>GHFKDPKRLYCKNGGFFLRIHPDGRVDGVREKSDPHIKLQLQAEERGVVSIKGVSANRYLAMKEDGRLLASKSVTDECFFFERLESNNYNTYRSRKYTSWYVALKRTGQYKLGSKTGPGQKAILFLPMSAKS[2x];>[2x]TDNTKPNRMPVAPYWTSPEKMEKKLHAVPAAKTVKFKCPSSGTPQPTLRWLKNGKEFKPDHRIGGYKVRYATWSIIMDSVVPSDKGNYTCIVENEYGSINHTYQLDVVERSPHRPILQAGLPANKTV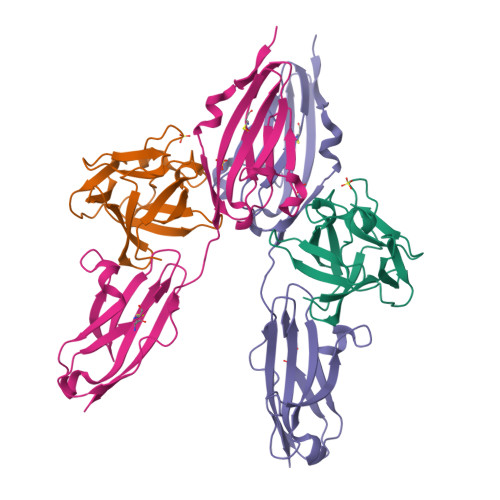ALGSNVEFMCKVYSDPQPHIQWLKHIEVNGSKIGPDNLPYVQILKTAGVNTTDKEMEVLHLRNVSFEDAGEYTCLAGNSIGLSHHSAWLTVLEALEER In Escherichia coli and numerous other bacteria, two of the principal enzymes mediating messenger RNA decay and RNA processing—RNase E, an endoribonuclease, and polynucleotide phosphorylase (PNPase), an exoribonuclease—assemble into a multi-enzyme complex known as the RNA degradosome. At the core of the assembly is the endoribonuclease RNase E, which initiates turnover of most messenger RNA (mRNA) transcripts and processes precursors of ribosomal RNAs, transfer RNAs, and small regulatory RNAs (sRNAs). Notwithstanding, PNPase predominantly acts as phosphorolytic 3′ → 5′ exoribonuclease that catalyses the processive degradation of single-stranded RNA, involved both in mRNA decay and sRNA-mediated gene regulation. Beyond the residues that form the catalytic core (1–529), each protomer of RNase E presents an intrinsically disordered C-terminal domain (CTD), extending from residues 530–1061, that serves as a scaffold for the RNA degradosome.

Purified RNase E 921–1061-muGFP peptide was combined in molar excess with the PNPase core, and the complex structurally characterized by cryo-EM. Several rounds of focused 3D-classification and focused 3D-refinement resulted in a cryo-EM map at overall 2.6 Å resolution, allowing an atomic model to be built for the PNPase core:RNase E complex using the automated model building tool ModelAngelo. The cryo-EM map is well-defined for the RNase E peptide from residue 1003 to residue 1057, therefore, only these residues were built in the atomic model. The model confirms the presence of the β-strand between residues 1048–1053 (β1 strand), and a second β-strand was identified and built, formed by the strongly conserved residues 1005 – 1008 (β2 strand), and similar to the residues forming β1 strand. 3D classification and 3D refinement confirmed that only one RNase E peptide engages with a PNPase trimer, interacting with two protomers, leaving the third ribonuclease protomer exposed and unoccupied. First, the β-strands resemble one another both in length, sequence and interaction pattern: His1005 on β2 strand and His1049 on β1 strand interact with the Asp328 present on the β-sheet of one PNPase protomer (Bix). In particular, Arg1056 form polar interactions with PNPase residues, namely Glu322 and Asp320. Each Arg in the two proline motifs, namely Arg1056 from the β1 motif (1053–1061) and Arg1012 from the β2 motif (1009–1017) form three salt bridges with different residues on PNPase, suggesting that Arg1012 and Arg1056 are key residues for the interaction with PNPase. On the other hand, the atomic model presented here reveals that the upstream region, from residues 1005 to 1039, forms several interactions with the two PNPase protomers engaged by RNase E peptide, which are not limited to the residues forming the β-strand or the proline motif.

>[3x]MLNPIVRKFQYGQHTVTLETGMMARQATAAVMVSMDDTAVFVTVVGQKKAKPGQDFFPLTVNYQERTYAAGRIPGSFFRREGRPSEGETLIARLIDRPIRPLFPEGFVNEVQVIATVVSVNPQVNPDIVAMIGASAALSLSGIPFNGPIGAARVGYINDQYVLNPTQDELKESKLDLVVAGTEAAVLMVESEAQLLSEDQMLGAVVFGHEQQQVVIQNINELVKEAGKPRWDWQPEPVNEALNARVAALAEARLSDAYRITDKQERYAQVDVIKSETIATLLAEDETLDENELGEILHAIEKNVVRSRVLAGEPRIDGREKDMIRGLDVRTGVLPRTHGSALFTRGETQALVTATLGTARDAQVLDELMGERTDTFLFHYNFPPYSVGETGMVGSPKRREIGHGRLAKRGVLAVMPDMDKFPYTVRVVSEITESNGSSSMASVCGASLALMDAGVPIKAAVAGIAMGLVKEGDNYVVLSDILGDEDHLGDMDFKVAGSRDGISALQMDIKIEGITKEIMQVALNQAKGARLHILGVMEQAINAPRGDIS;> NHATAPMTRAPAPEYVPEAPRHSDWQRPTFAFEGKGAAGGHTATHHASAAPARPQPVE>RICFNHQTSQPQTTKTC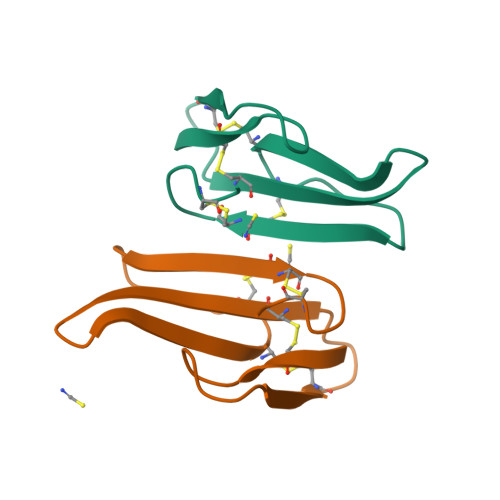SPGESSCYNKQWSDFRGTIIERGCGCPTVKPGIKLSCCESEVCNN[2x]> GDWLDLNTTSSVETGQAIVTLDDAQIALNGIYRLASGHSYYGDNYWYYGDCRAADVQARITKGDGKRVSPYYEYNVLASDNLNIVLPWNTVYKVIRQTNNLIQKIESG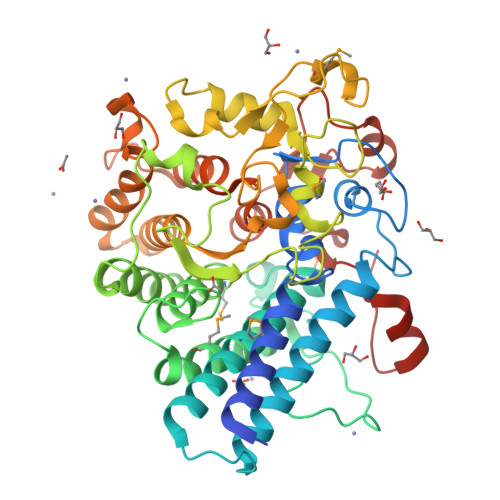SIQSSDTKELNRIKSEALVMRGLSLFNLTRLFGMPYTNDKGASLGVPIETSPSDPTHKPSRSTVAQCYEQVVSDMSNALSGLRQETSNGYINYWAAQALLSRVYLNMGEYQKAYDAATDVIKNNGGRYQLYSYEEYPNVWGQDFQSESLFELYITLSEPSGGTGGEGAPMVYANEATVDWNNLILSEDFLNLLNEDPKDVRHCLTKESVIENNTGLPAAAMHEKVYLAKFPGKTGDDPKTNNICIIRLSEVYLNAAEAGLKKGTDIEEAQGYLNDIISRRTTDTSQQVSTETFTLDRILKERRKELVGEGEVFYDYLRNGLAIERKGSWHLETLKASNAQKIEATDLRIALPIPQSEIDANPNIQQNPR> ACACTACAATGTTGCAAT;> GTATTGC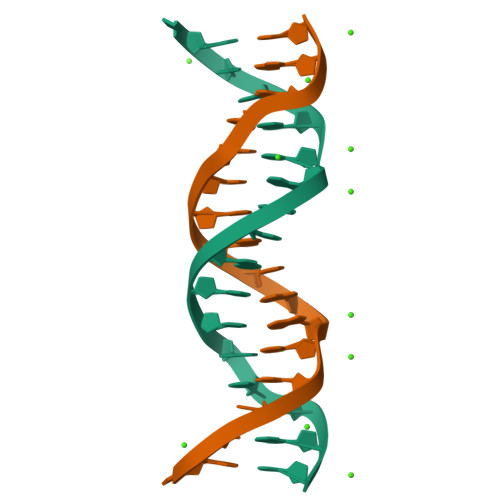AACATTGTAGT We also solved the crystal structure of BmTrxR, being the first crystallographic structure of a TrxR from a nematode, which, surprisingly, is a fusion of a large TrxR domain with a Grx-like domain at the N-terminus lacking a typical Grx active site motif. Helminth TrxRs are members of the high molecular weight TrxR subfamily and are selenocysteine (Sec, U)-containing homodimeric flavoenzymes. They transfer reducing equivalents from NADPH to their flavin adenine dinucleotide (FAD) cofactor and, subsequently, to a pair of cysteines located at the si-face of the isoalloxazine ring. From there, electrons are transferred to the mobile Sec-containing C-terminal redox center of the symmetrical subunit, that, upon reduction of its Cys-Sec motif, reaches the solvent-exposed surface of the enzyme transferring electrons to the incoming oxidized Trx.

Auranofin is a gold-containing compound in which the Au(I) is tethered between a thioglucose and a triethylphosphine with a linear geometry. It is a well-known selenocysteine-cysteine interacting compound. Crystals of BmTrxR, were soaked with 500 μM NADPH and 4–5 equivalents of auranofin for 72 h, and the resulting structure was solved by molecular replacement at 3.1 Å. After the refinement process and geometry optimization of the model, an anomalous difference Fourier map was calculated from 40 to 3.1 Å and contoured at 7 σ. Its superimposition on the difference density map (Fo - Fc) contoured at the same σ and calculated on the refined BmTrxR structure without the metal, clearly shows the position of the gold atoms in the asymmetric unit; an electron density associated with the anomalous signal of a gold atom is present on C22 of subunit b. The gold atom is found at the expected distance for a Au–S bond (2.3 Å) with additional electron density detected from the other side of Au(I) with respect to C22. However, the low resolution of the structure and the incomplete occupancy of the metal (∼50%) prevented identification of the ligand. As expected, auranofin, a pan-TrxR inhibitor, also capable of targeting SmTGR, was here found to efficiently inhibit also BmTrxR and OvTrxR.

>[3x]MSPIPNRVSSGSLADAVFKSACEERILLAYADYNPDMTKVVNLFSKYNETVNTVRVSNDAVKDILEIVGWPSMPLIFVKGNCCGGFKELYQLEESGFLNEWLKEHEYDLAIVGGGSGGLAAAKEAVRLGKKVVCLDFVKPSAMGTTWGLGGTCVNVGCIPKKLMHQAALLGEYIEDAKKFGWEIPEGAIKLNWHQLKNAVQNHIASLNWGYRVQLKEKSVTYMNSYATFTGSHELSVKNKKGKVEKVTADRFLIAVGLRPRFPDVPGALECCISSDDLFSLPYNPGKTLCVGASYVSLECAGFLKGIGNDVTVMVRSVLLRGFDQDMAERIKKHMTERGVKFVQCVPIKYERLKKPTDSEPGMIRVHTMQEDEDGTKEVTEDFNTVLMAIGRDAMTDDLGLDVVGVNRAKSGKIIGRREQSVSCPYVYAIGDVLYGSPELTPVAIQAGKVLMRRLFTGSSELTEYDKIPTTVFTPLEYGSCGLSEYSAIQKYGKENINVYHNVFIPLEYAVTERKEKTHCYCKLICLKNEQDLILGFHILTPNAGEITQGFAIALKFDAKKADFDRLIGIHPTVAENFTTLTLVKEDGQTLKATGCUG>[6x]EHVTGKWFSVPELRLRDHRFIVPLDYSKSSPKITVFAREIVAVGKEEQAMPYLLYLQGGPGFEGPRPSEASGWIQRACEEFRVVLLDQRGTGLSTPLTCSSMLQFK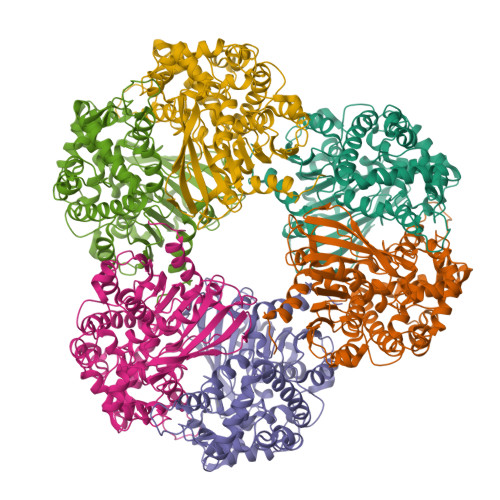SAKELADYLVHFRADNIVKDAEFIRVRLVPKADPWTILGQSFGGFCALTYLSFAPEGLKQVLITGGIPPIGKACTADDVYEAGFEQVARQNEKYYKRFPQDIEIVRELVNYLAESEGGGVPLPSGGILTPKGLQTLGLSGLGSSTGFERLHYMLERVWDPILVTGAPKCISQFFLNAFESWHSFDTNPLYALLHEAIYCEGASSGWSAHRLRDKYEYKFDAMKAVKESQPVLFTGEMIFPWMFDEIHALKPFKAAADLLAKKEDWPPLYDVPRLQNNKVPVAAAVYYEDMYVNFKLVTETASHISGIRLWVTNEFMHSGLRDAGRQIIDHLLGMINGKKPLF>[8x]MEIKRRTQEERSAATREALITGARKLWGLRGYAEVGTPEIATEAGVTRGAMYHQFADKAALFRDVVEVVEQDVMARMATLVAASGAATPADAIRAAVDAWLEVSGDPEVRQLILLDAPVVLGWAGFRDVAQRYSLGMTEQLITEAIRAGQLARQPVRPLAQVLIGALDEAAMFIATADDPKRARRETRQVLRRLIDGMLNGKLAAALEHHHHHH

Here, we show cytokinins induced the strong expression of the M. tuberculosis gene Rv0077c. We found that Rv0077c expression is repressed by a TetR-like transcriptional repressor, Rv0078. As previously reported, Rv0078 forms dimers resembling other TetR-like proteins. Rv0078 has an N-terminal DNA-binding domain (DBD) and a C-terminal ligand-binding domain (LBD).

The estimated stoichiometry of DNA duplex to Rv0078 dimer was 0.66, suggesting that two Rv0078 dimers bind to one operator sequence. As predicted by the ITC experiments, we observed two Rv0078 dimers bound to a DNA duplex where each dimer bound on opposite sides of the DNA. The top or “central” dimer bound the DNA palindrome symmetrically, while the bottom or “peripheral” dimer bound to DNA off-center, staggered from the central dimer binding site by 7 bp. Thus, the longer-than-canonical (i.e., tetO) binding site is required for accommodation of two Rv0078 dimers, unlike TetR, which binds to tetO as a single dimer. DNA binding induced significant conformational changes across the Rv0078 dimer structure, with a root mean square deviation (RMSD) of 2.13 Å compared to the DNA-free dimer. In particular, the two α3 helices move toward each other by ~6 Å, in order to reduce their distance to 36.4 Å and fit in the DNA major grooves. It appears that changes initiated in the DBD regions upon binding to the DNA are transmitted to the LBD via the DBD-LBD interface, which involves extensive interactions, including two salt bridges and six H-bonds. Specifically, the hydroxyl groups of Thr37, Thr47, and Tyr52 interacted strongly with DNA phosphates at a distance of 2.6 Å. Arg48 is the only residue that interacted with DNA by recognizing a guanine base at a distance of 2.6 Å.> MIEAPDVKPWLFLIKPYEGESLSHFLGRFRRANH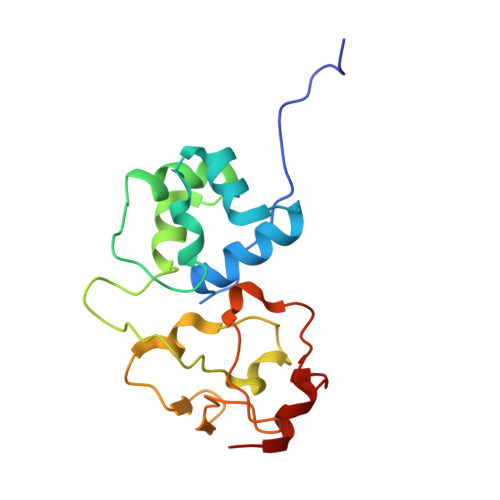LSASGLGTLAGIGAIVARWERFHFNPRPSQQELEAIASVVEVDAQRLAQMLPPAGVGMQHEPIRLCGACYAESPCHRIEWQYKSVWKCDRHQLKILAKCPNCQAPFKMPALWEDGCCHRCRMPFAEMAKLQKV>MRGSHHHHHHGSACQNLNGKVAFVTGGSRGIGAAIVRRLAADGADIAFTYVSASSKNVATALVQELEAKGRRARAIQADSADPAQVRQAVEQAIVQLGPVDVLVNNAGIFLAGPLGEVTLDDYERTMNINVRAPFVAIQAAQASMPDGGRIINIGSCLAERAGRAGVTLYAASKSALLGMTRGLARDLGARGITANVVHPGPIDTDM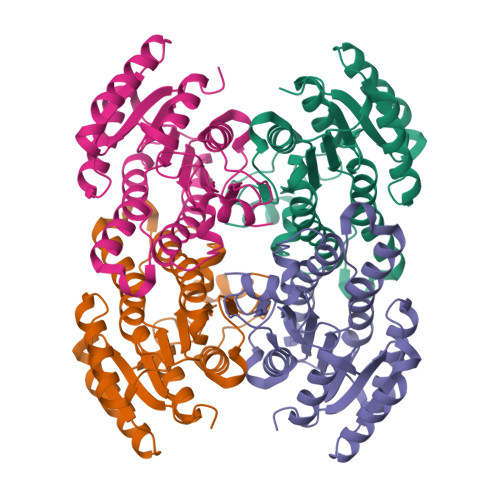NPADGERSGELVAVLSLPHYGEVRDIAGMVAFLAGPDGRYVTGASLAVDGGFAA[4x]>[6x]MGSSHHHHHHSSGLVPRGSHVTDTDLITAGESTDGKPSDAAATDPPDLNADEPAGSLATMVLPELRALANRAGVKGTSGMRKNELIAAIEEIRRQANGAPAVDRSAQEHDKGDRPPSSEAPATQGEQTPTEQIDSQSQQVRPERRSATREAGPSGSGERAGTAADDTDNRQGGQQDAKTEERGTDAGGDQGGDQQASGGQQARGDEDGEARQGRRGRRFRDRRRRGERSGDGAEAELREDDVVQPVAGILDVLDNYAFVRTSGYLPGPHDVYVSMNMVRKNGMRRGDAVTGAVRVPKEGEQPNQRQKFNPLVRLDSINGGSVEDAKKRPEFGKLTPLYPNQRLRLETSTERLTTRVIDLIMPIGKGQRALIVSPPKAGKTTILQDIANAITRNNPECHLMVVLVDERPEEVTDMQRSVKGEVIASTFDRPPSDHTSVAELAIERAKRLVEQGKDVVVLLDSITRLGRAYNNASPASGRILSGGVDSTALYPPKRFLGAARNIEEGG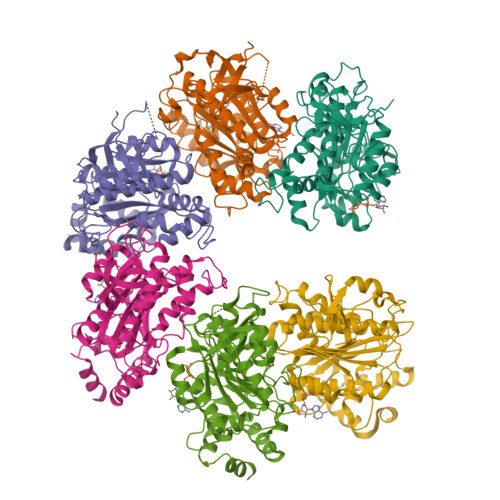SLTIIATAMVETGSTGDTVIFEEFKGTGNAELKLDRKIAERRVFPAVDVNPSGTRKDELLLSPDEFAIVHKLRRVLSGLDSHQAIDLLMSQLRKTKNNYEFLVQVSKTTPGSMDSD>[2x]MGQGNDTSEVMLLDTGWEFSQSGTEKWMPATVPGTVHQDLISHELLPNPFYGMNEKKIQWVENEDWEYRTSFIVSEEQLNRDGIQLIFEGLDTYADVYLNGSLLLKADNMFVGYTLPVKSVLRKGENHLYIYFHSPIRQTLPQYASNGFNYPADNDHHEKHLSVFSRKAPYSYGWDWGIRMVTSGVWRPVTL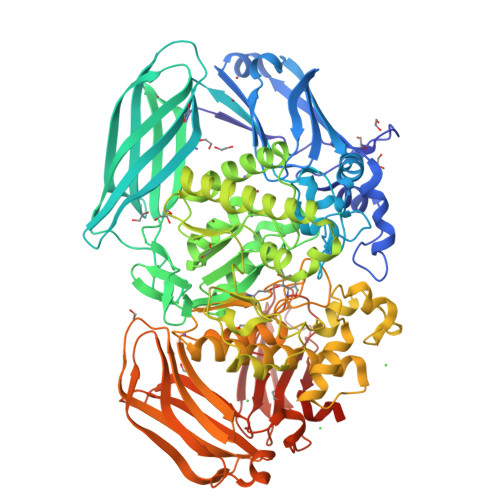RFYDIATISDYYVRQLSLTDENARLSNELIVNQIVPQKIPAEVRVNVSLNGTTVTEVKQQVTLQPGINHITLPAEVTNPVRWMPNGWGTPTLYDFSAQIACGDRIVAEQSHRIGLRTIRVVNEKDKDGESFYFEVNGIPMFAKGANYIPQDALLPNVTTERYQTLFRDMKEANMNMVRIWGGGTYENNLFYDLADENGILVWQDFMFACTPYPSDPTFLKRVEAEAVYNIRRLRNHASLAMWCGNNEILEALKYWGFEKKFTPEVYQGLMHGYDKLFRELLPSTVKEFDSDRFYVHSSPYLANWGRPESWGTGDSHNWGVWYGKKPFESLDTDLPRFMSEFGFQSFPEMKTIAAFAAPEDYQIESEVMNAHQKSSIGNSLIRTYMERDYIIPESFEDFVYVGLVLQGQGMRHGLEAHRRNRPYCMGTLYWQLNDSWPVVSWSSIDYYGNWKALHYQAKRAFAPVLINPIQQNDSLSVYLISDRLDTMEQMTLEMKVVDFDGKTLGKKIQVHSLEVPANTSKCVYRAKLDGWLTPEDCRRSFLKLILKDKSGHQVAESVHFFRKTKDLQLPPTSVSYQMKQTDGKCELTLFSSMLAKDIFIETPLQGARYSDNFFDLLPGERKKVIITSPRIKKGEELPVNIKHIRETYKLEHHHHHH> MEEIQGY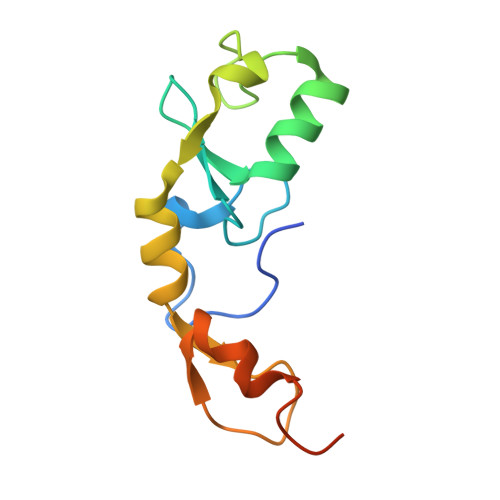DVEFDPPLESKYECPICLMALREAVQTPCGHRFCKACIIKSIRDAGHKCPVDNEILLENQLFPDNFAKREILSLMVKCPNEGCLHKMELRHLEDHQAHCEFALLEHHHHHH>EFPEITEEMEKEIKNVFRNGNQDEVLSEAFRLTITRKDIQTLNHLNWLNDEIINFYMNMLMERSKEKGLPSVHAFNTFFFTKLKTAGYQAVKRWTKKVDVFSVDILLVPIHLGVHWCLAVVDFRKKNITYYDSMGGINNEACRILLQYLKQESIDKKRKEFDTNGWQLFSKKSQEIPQQMNGSDAGMFACKYADCITKDRPINFTQQHMPYFRKRMVWEILHRKLL[2x];>EYIKLKVIGQDSSEIHFKVKMTTHLKKLKESYCQRQGVPMNSLRFLF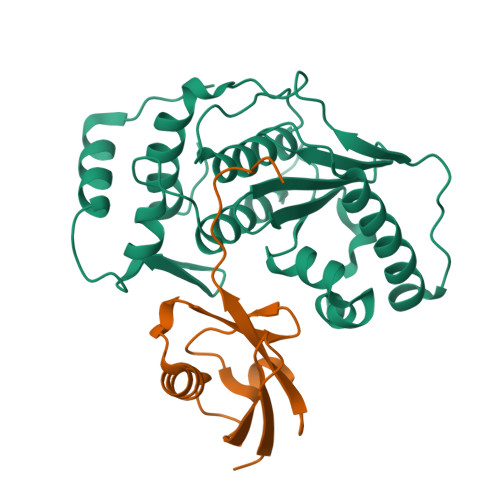EGQRIADNHTPKELGMEEEDVIEVYQEQTGGHSTVC[2x]Crocagins (1 and 2)24 are very small, intriguing RiPPs that possess a tetracyclic ring system, which consists of a pyrroloindoline fused to a tetrahydropyrimidinone moiety. Here we use in vitro experiments to demonstrate that three proteins, CgnB, CgnC and CgnE, are sufficient for the production of the hallmark tetracyclic crocagin core from the precursor peptide CgnA. We further show that the hydrolase CgnD liberates the crocagin core scaffold, which is subsequently N-methylated by CgnL. The crystal structures of the homologues CgnB and CgnE reveal them to be the founding members of a peptide-binding protein family and allow us to rationalize their distinct functions.

First, the structure of CgnE was determined to 2.0 Å. In CgnE, the metal binding site of Zn2+ 1 was disrupted by mutations in two metal-coordinating residues (CgnB numbering), Glu274Lys and His280Tyr, and no density for metal ions was observed in the CgnE structure. As expected for homologous proteins, the Cα root-mean-square deviation (r.m.s.d.) between the structures of CgnB and CgnE was only 1.2 Å over 284 residues. The aminopeptidases form an extensive dimer interface, and the residues involved in its formation are largely missing in CgnB and CgnE, which rationalizes their monomeric state in the crystals. The leader peptide is enriched with positively charged amino acids, and both CgnB and CgnE show a large, strongly negatively charged patch near the possible binding site. We found the binding of CgnE to the CgnALP to be almost 300 times weaker than binding to CgnA (KD = 514 µM). The main driver for binding thus appears to be the core peptide, and it is tempting to suggest that CgnE’s role may be to recruit the substrate peptide to CgnC and present the core peptide in a particular way that enables or accelerates correctly timed catalysis. CgnE appears to recruit the substrate peptide CgnA to CgnC and assist in catalysis, perhaps by presenting the core peptide in a specific conformation or by ensuring appropriate timing of the hydroxylation reactions, but does not seem to possess catalytic activity itself.

>[2x]GMGGRRTIGIRSGEGAIMNASDFYALLRGRGMPVVVDDAEAAAVVSELGFRTVPFEAFDFDSPSEDPALVIVAQMGNVDALHGLWERSGTPLMHLALAKFDGGLSRLRAGLARVLAVDTDAALKRRAEAYEQLFSSASVEIASGEGVLRCHIGDEVEVGNCGDTLEQGFLYSVAEFLEASVVNLEGERSTFWVEGELPFDGFIHLSNSAALKERWGGMLDEFMRRSREGANLVRFADNVIDRLVVGGVDVTSALAGLSQGEERGMAATEFGLGCADAEAAEPFGVNSLLHKSAGGAYIGIGKGLRIPHIDFIARGATIRFIPAAEG> GUGUGCCCGGCAUGGGUGCAGUCUAUAGGGUGAGAGUCCCGAACUGUGAAGGCAGAAGUAACAGUUAGCCUAACGCAAGGGUGUCCGUGGCGACAUGGAAUCUGAAGGAAGCGGACGGCAAACCUUCGGUCUGAGGAACACGAACUUCAUAUGAGGCUAGGUAUCAAUGGAUGAGUUUGCAUAACAAAACAAAGUCCUUUCUGCCAAAGUUGGUACAGAGUAAAUGAAGCAGAUUGAUGAAGGGAAAGACUGCAUUCUUACCCGGGGAGGUCUGGAAACAGAAGUCAGUAGAAGUCAUAGUACCCUGUUCGCAGGGGAAGGACGGAACAAGUAUGGCGUUCGCGCCUAAGCUUGAACUGCCGUAUACCGAACGGUACGUACGGUAGUGUG;> GGGGUUA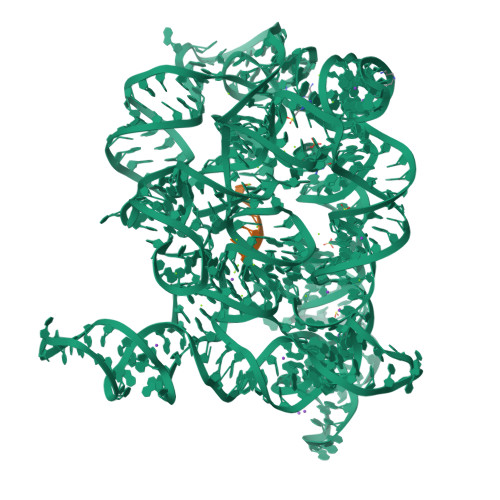U>[2x]MKGTIVGTWIKTLRDLYGNDVVDESLKSVGWEPDRVIT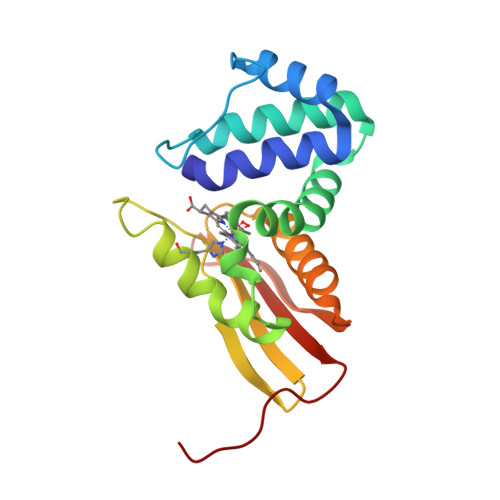PLEDIDDDEVRRIFAKVSEKTGKNVNEIWREVGRQNIKTLSEWFPSYFAGRRLVNFLMMMDEVHLQLTKMIKGATPPRLIAKPVAKDAIEMEYVSKRKMYDYFLGLIEGSSKFFKEEISVEEVERGEKDGFSRLKVRIKFKNPVFEYKKN Many proteins, including the EP300/CBP histone acetyltransferases (HATs), contain several targetable domains. EP300 and CBP broadly regulate the activity of other proteins through their protein acetyltransferase catalytic activity. These proteins contain several highly homologous domains, including KIX, bromodomains (BRDs) and HAT domains, through which they interact with, dock to, and acetylate target proteins, respectively. EP300/CBP are critical gene-regulatory targets in cancer, with existing high potency inhibitors of either the catalytic HAT domain or protein-binding bromodomain (BRD). Using crystallography, we identify the binding mechanism of the EP300/CBP-specific BRD inhibitor CCS1477 in complex with the EP300, CBP and BRD4 BRDs, and define components of the CCS1477 catalytic binding core that are required for compound activity.

To understand the structural basis for the observed differential binding affinities of CCS1477 between EP300/CBP and BRD4, we next solved the co-crystal structures of the respective bromodomains with CCS1477. As expected, CCS1477 binds through canonical hydrogen-bonding interactions of its dimethyl isoxazole moiety with a conserved asparagine residue in the acetyl-lysine (Kac) binding site (CBPN1168, EP300N1132, BRD4N140). A major difference, however, between the inhibitor binding pattern in EP300/CBP and BRD4 is the involvement of an arginine side chain (EP300R1137, CBPR1173) that interacts with the difluorophenyl ring of CCS1477 through Pi-cation interactions, while establishing an additional hydrogen-bond with the piperidinone oxygen. In EP300/CBP, an analogous tryptophan residue is not present, and instead the equivalent LPF shelf is less bulky and facilitates interaction with CCS1477. Superposition of CCS1477 as bound in the respective Kac sites reveals an altered binding pose, reflecting the reduced shape complementarity between CCS1477 and BRD4, as compared with EP300/CBP. CCS1477 produced a greater thermal shift with EP300 or CBP, as compared with BRD4. Further analysis of the binding energies by isothermal titration calorimetry (ITC) confirmed significantly stronger interaction of CCS1477 with the bromodomains of CBP and EP300 (Kd = 4.0 and 26 nM, respectively) than with BD1 of BRD4 (Kd = 403 nM). Thus, CCS1477 displays preferential binding to the bromodomains of EP300 and CBP, compared with BRD4. Lysates were treated with biotinylated-CCS1477 at 1 or 10 μM, prior to western blotting. These data demonstrated that at lower concentrations, biotinylated-CCS1477 interacted with EP300 but not BRD4. Thus, the difluorophenyl group is a critical moiety in the CCS1477 pharmacophore that facilitates potent interaction with the bromodomain of EP300/CBP and is required for efficacy in cell line models of G3MB.

>[2x]IFKPEELRQALMPTLEALYRQDPESLPFRQPVDPQLLGIPDYFDIVKSPMDLSTIKRKLDTGQYQEPWQYVDDIWLMFNNAWLYNRKTSRVYKYCSKLSEVFEQEIDPVMQSLG> GSHMASMKKKGSVVIVGRINLSGDTAYAQQTRGEEGCQETSQTGRDKNQVEGEVQIVST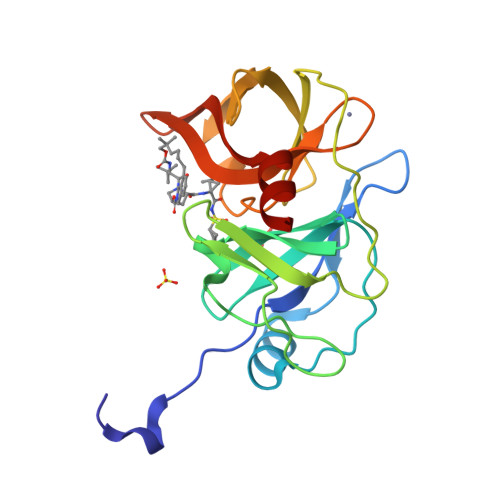ATQTFLATSINGVLWTVYHGAGTRTIASPKGPVTQMYTNVDKDLVGWQAPQGSRSLTPCTCGSSDLYLVTRHADVIPVRRRGDSRGSLLSPRPISYLKGSAGGPLLCPAGHAVGIFRAAVSTRGVAKAVDFIPVESLETTMRSP> MGDAPSPEEKLHLITRNLQEVLGEEKLKEILKERELKIYWRTATTGKPHVAYFVPMSKIADFLKAGCEVTILFADLHAYLDNMKAPWELLELRVSYYENVIKAMLESIGVPLEKLKFIK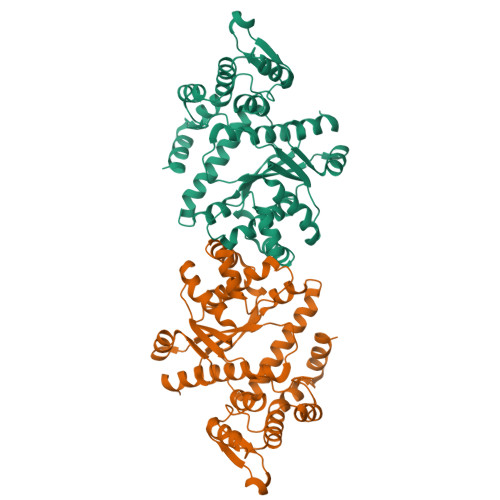GTDYQLSKEYTLDVYRLSSVVTQHDSKKAGAEVVKQVEHPLLSGLLYPGLQALDEEYLKVDAQFGGIDQRKIFTFAEKYLPALGYSKRVHLMNPMVPGLTGSKMSSSEEESKIDLLDRKEDVKKKLKKAFCEPGNVENNGVLSFIKHVLFPLKSEFVILRDEKWGGNKTYTAYVDLEKDFAAEVVHPGDLKNSVEVALNKLLDPIREKFNTPALKKLASAAYPDPSKQKPMAKGPAKNSEPEEVILEHHHHHH>[2x]MWDVIDLSRWQFALTALYHFLFVPLTLGLIFLLAIMETIYVVTGKTIYRDMTRFWGKLFGINFALGVATGLTMEFQFGTNWSFYSNYVGDIFGAPLAMEALMAFFLESTFVGLFFFGWQRLNKYQHLLVTWLVAFGSNLSALWILNANGWMQYPTGAHFDIDTLRMEMTSFSELVFNPVSQVKFVHTVMAGYVTGAMFIMAISAWYLLRGRERNVALRSFAIGSVFGTLA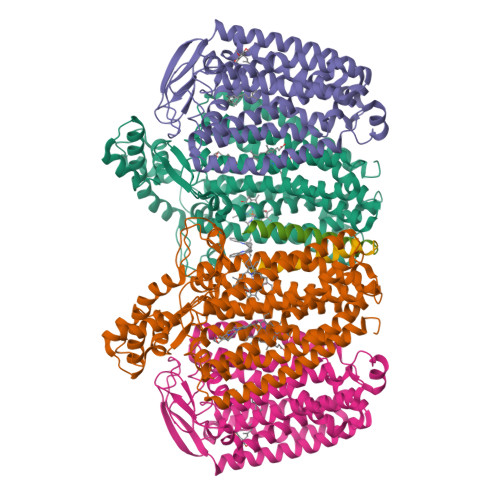IIGTLQLGDSSAYEVAQVQPVKLAAMEGEWQTEPAPAPFHVVAWPEQDQERNAFALKIPALLGILATHSLDKPVPGLKNLMAETYPRLQRGRMAWLLMQEISQGNREPHVLQAFRGLEGDLGYGMLLSRYAPDMNHVTAAQYQAAMRGAIPQVAPVFWSFRIMVGCGSLLLLVMLIALVQTLRGKIDQHRWVLKMALWSLPLPWIAIEAGWFMTEFGRQPWAIQDILPTYSAHSALTTGQLAFSLIMIVGLYTLFLIAEVYLMQKYARLGPSAMQSEQPTQQQG;>[2x]MFDYETLRFIWWLLIGVILVVFMISDGFDMGIGCLLPLVARNDDERRIVINSVGAHWEGNQVWLILAGGALFAAWPRVYAAAFSGFYVAMILVLCSLFFRPLAFDYRGKIADARWRKMWDAGLVIGSLVPPVVFGIAFGNLLLGVPFAFTPQLRVEYLGSFWQLLTPFPLLCGLLSLGMVILQGGVWLQLKTVGVIHLRSQLATKRAALLVMLCFLLAGYWLWVGIDGFVLLAQDANGPSNPLMKLVAVLPGAWMNNFVESPVLWIFPLLGFFCPLLTVMAIYRGRPGWGFLMASLMQFGVIFTAGITLFPFVMPSSVSPISSLTLWDSTSSQLTLSIMLVIVLIFLPIVLLYTLWSYYKMWGRMTTETLRRNENELY;>[2x]MWYLLWFVGILLMCSLSTLVLVWLDPRLKS> ACTKNAIAQTGFNKDKYFNGDVWYVTDYLDLEPDDVPKRYCAALAAGTASGKLKEALYHYDPKTQDTFYDVSELQVESLGKYTANFKKVDKNGNVKVAVTAGNYYTFTVMY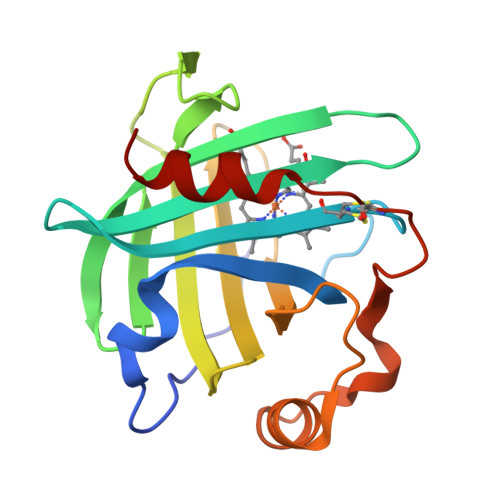ADDSSALIHTCLHKGNKDLGDLYAVLNRNKDAAAGDKVKSAVSAATLEFSKFISTKENNCAYDNDSLKSLLTK tridec-12-en-2-one | C13 H24 O | 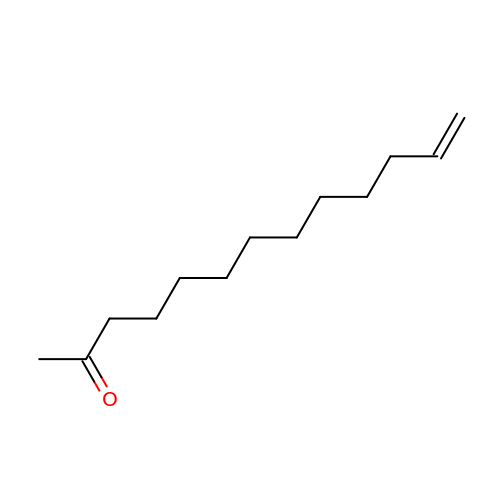UYCZPLKICNDOCL-UHFFFAOYSA-N> GGCGUGGUUGACACGCAGACCUCUUACAAGAGUGUCUAGGUGCCUUUGAGAGUUACUCUUUGCUCUCUUCGGAAGAACCCUUAGGGGUUCGUGCAUGGGCUUGCAUAGCAAGUCUUAGAAUGCGGGUACCGUACAGUGUUGAAAAACA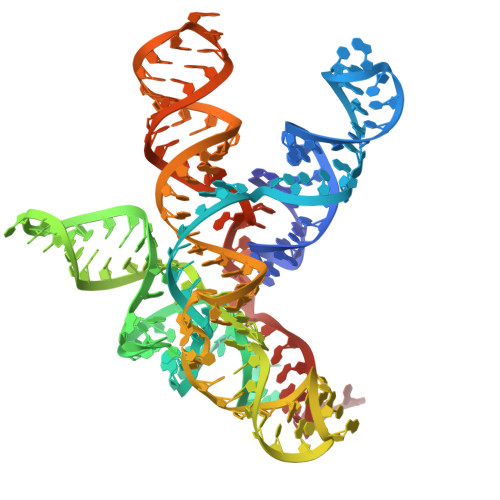CUGUAAAUCUCUAAAAGAGACCA> MKCHRCGSDNVRKMVDSPVGDAWEVYVCEKCCYSWRSTENPVVMEKFKLDDNKIAN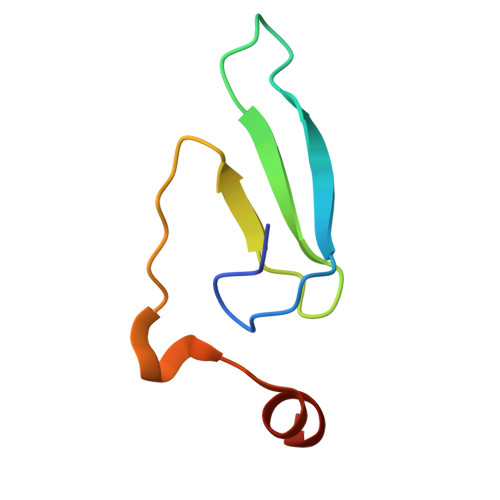MG>XSSDPLVVAANIIGILHLILWIL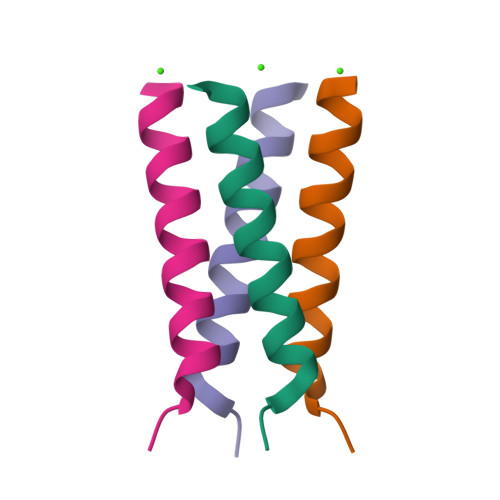DRLX[8x]>MQSSVNEFLTPRHIDVQVVSQTRAKITLEPLERGFGHTLGNALRRILLSSMPGCAVVEAEIDGVLHEYSAIEGVQEDVIEILLNLKGLAIKLHGRDEVTLTLAKKGSGVVTAADIQLDHDVEIINGDHVIANLADNGALNMKLKVARGRGYEPADARQSDEDESRSIGRLQLDASFSPVRRVSYVVENARVEQRTNLDKLVLDLETNGTLDPEEAIRRAATILQQQLAAFVDLKGDSEPVVEEQEDEIDPILLRPVDDLELTVRSANCLKAENIYYIGDLIQRTEVELLKTPNLGKKSLTEIKDVLASRGLSLGMRLDNWPPASLKKDDKATA[2x];> MAYSYTEKKRIRKDFSKLPDVMDVPYLLAIQLDSYREFLQAGATKEQFRDVGLHAAFKSVFPIISYSGNAALEYVGYRLGEPAFDVKECVLRGVTFAVPLRVKVRLIIFDRESSNKAIKDIKEQEVYMGEIPLMTENGTFIINGTERVIVSQLHRSPGVFFDHDRGKTHSSGKLLYSARIIPYRGSWLDFEFDPKDCVFVRIDRRRKLPASVLLRALGYSTEEILNAFYATNVFHIKGETLNLELVPQRLRGEVASIDIKDGSGKVIVEQGRRITARHINQLEKAGVSQLEVPFDYLIGRTIAKAIVHPATGEIIAECNTELTLDLLAKVAKAQVVRIETLYTNDIDCGPFISDTLKIDNTSNQLEALVEIYRMMRPGEPPTKEAAETLFGNLFFSAERYDLSAVGRMKFNRRIGRTEIEGPGVLSKEDIIDVLKTLVDIRNGKGIVDDIDHLGNRRVRCVGEMAENQFRVGLVRVERAVKERLSMAESEGLMPQDLINAKPVAAAIKEFFGSSQLSQFMDQNNPLSEITHKRRVSALGPGGLTRERAGFEVRDVHPTHYGRVCPIETPEGPNIGLINSLATYARTNKYGFLESPYRVVKDSLVTDEIVFLSAIEEADHVIAQASATLNEKGQLVDELVAVRHLNEFTVKAPEDVTLMDVSPKQVVSVAASLIPFLEHDDANRALMGSNMQRQAVPTLRADKPLVGTGMERNVARDSGVCVVARRGGVIDSVDASRVVVRVADDEVETGEAGVDIYNLTKYTRSNQNTCINQRPLVSKGDVVARGDILADGPSTDMGELALGQNMRVAFMPWNGFNFEDSICLSERVVQEDRFTTIHIQELTCVARDTKLGPEEITADIPNVGEAALNKLDEAGIVYVGAEVQAGDILVGKVTPKGETQLTPEEKLLRAIF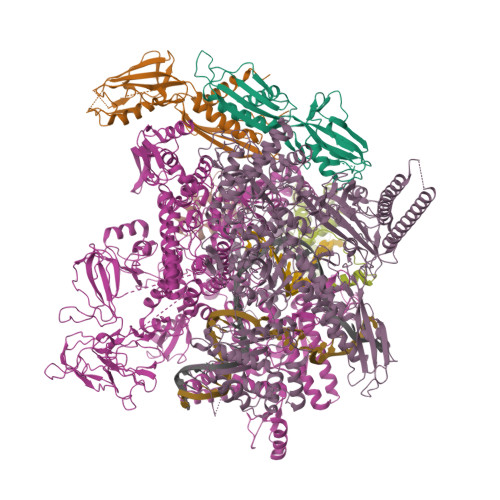GEKASDVKDTSLRVPTGTKGTVIDVQVFTRDGVERDSRALSIEKMQLDQIRKDLNEEFRIVEGATFERLRAALVGAKAEGGPALKKGTEITDDYLDGLERGQWFKLRMADDALNEQLEKAQAYISDRRQLLDDKFEDKKRKLQQGDDLAPGVLKIVKVYLAIKRRIQPGDKMAGRHGNKGVVSVIMPVEDMPHDANGTPVDIVLNPLGVPSRMNVGQILETHLGLAAKGLGEKINRMLEEQRKVAELRKFLHEIYNEIGGREENLDELGDNEILALAKNLRGGVPMATPVFDGAKEREIKAMLKLADLPESGQMRLFDGRTGNQFERPTTVGYMYMLKLNHLVDDKMHARSTGSYSLVTQQPLGGKAQFGGQRFGEMEVWALEAYGAAYTLQEMLTVKSDDVNGRTKMYKNIVDGDHRMEAGMPESFNVLIKEIRSLGIDIELETE;> MKDLLNLLKNQGQIEEFDAIRIGLASPEMIRSWSFGEVKKPETINYRTFKPERDGLFCAKIFGPVKDYECLCGKYKRLKHRGVICEKCGVEVALAKVRRERMGHIELASPVAHIWFLKSLPSRIGLLLDMTLRDIERVLYFESYVVIDPGMTTLEKGQLLNDEQYFEALEEFGDDFDARMGAEAVHELLNAIDLEHEIGRLREEIPQTNSETKIKKLSKRLKLMEAFQGSGNKPEWMVLTVLPVLPPDLRPLVPLDGGRFATSDLNDLYRRVINRNNRLKRLLDLAAPDIIVRNEKRMLQEAVDALLDNGRRGRAITGSNKRPLKSLADMIKGKQGRFRQNLLGKRVDYSGRSVITVGPTLRLHQCGLPKKMALELFKPFIFGKLEGRGMATTIKAAKKMVERELPEVWDVLAEVIREHPVLLNRAPTLHRLGIQAFEPVLIEGKAIQLHPLVCAAYNADFDGDQMAVHVPLTLEAQLEARALMMSTNNILSPANGEPIIVPSQDVVMGLYYMTREAINAKGEGMAFADLQEVDRAYRSGQASLHARVKVRINEKIKGEDGQLTANTRIVDTTVGRALLFQVVPAGLPFDVVNQSMKKKAISKLINHCYRVVGLKDTVIFADQLMYTGFAYSTISGVSIGVNDFVIPDEKARIINAATDEVKEIESQYASGLVTQGEKYNKVIDLWSKANDEVSKAMMANLSKEKVVDREGKEVDQESFNSMYMMADSGARGSAAQIRQLAGMRGLMAKPDGSIIETPITANFREGLNVLQYFISTHGARKGLADTALKTANSGYLTRRLVDVAQDLVVTEIDCGTEHGLLMSPHIEGGDVVEPLGERVLGRVIARDVFKPGSDEVIVPAGTLIDEKWVDFLEVMSVDEVVVRSPITCETRHGICAMCYGRDLARGHRVNIGEAVGVIAAQSIGEPGTQLTMRTFHIGGAASRTSAADNVQVKNGGTIRLHNLKHVVRADGALVAVSRSGELAVADDFGRERERYKLPYGAVISVKEGDKVDPGAIVAKWDPHTHPIVTEVDGTVAFVGMEEGITVKRQTDELTGLTNIEVMDPKDRPAAGKDIRPAVKLIDAAGKDLLLPGTDVPAQYFLPANALVNLTDGAKVSIGDVVARIPQETSKTRDITGGLPRVADLFEARRPKEPSILAEISGTISFGKETKGKRRLVITPNDGSDPYEELIPKWRHLNVFEGEQVNRGEVISDGPSNPHDILRLLGVSSLAKYIVNEIQDVYRLQGVKINDKHIETILRQMLRKVEVSESGDSSFIKGDQVELTQVLEENEQLGTEDKFPAKYERVLLGITKASLSTESFISAASFQETTRVLTEAAVTGKRDFLRGLKENVVVGRLIPAGTGLAYHSERKRQRDLGKPQRVSASEAEAALTEALNSSGN;> MARVTVEDCLDNVDNRFELVMLATKRARQLATGGKEPKVAWENDKPTVVALREIASGLVDENVVQQEDIVEDEPLFAAFDDEANTEAL;> MFQSTEQALAVAYWMFEQQPGPRSSTAMVIDSLRERFDRRFIERLPSGLSPHEWQAQAVMTVRFAQRQLAAHPLELAVVRAEFARGRDFVLGLAALRDWLKPAAGPIEQRAALALLMRMFRRPPSSIREIERLSGLSKSTLHRWDKEWRERVAALLRQALLRLEEPMAQVGIVCEH>[2x]EYGYIVTDQKP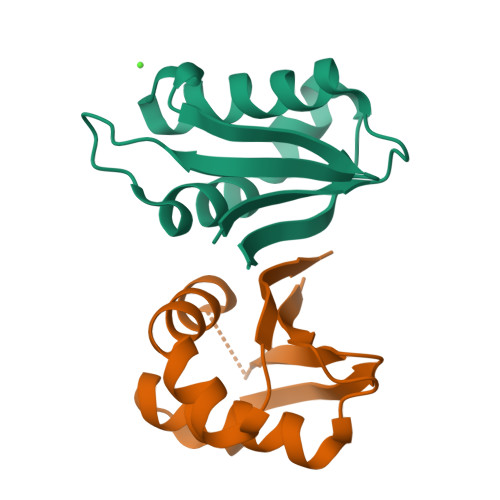LSLAAGVKLLEILAEHVHMSSGSFINIAVVGPALTFRIRHNEQNLSLADVTQQAGLVKSELEAQTGLQILQTGVGQRE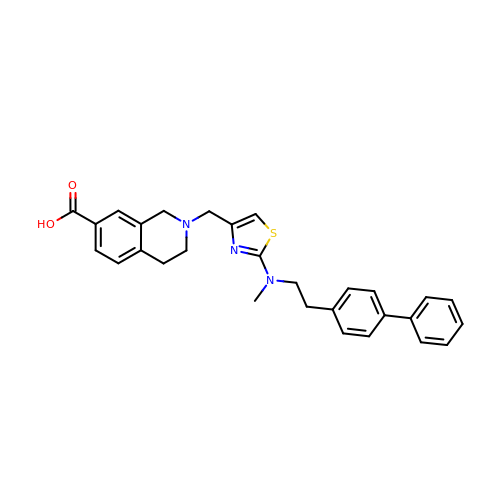2-[[2-[methyl-[2-(4-phenylphenyl)ethyl]amino]-1,3-thiazol-4-yl]methyl]-3,4-dihydro-1~{H}-isoquinoline-7-carboxylic acid | C29 H29 N3 O2 S | PZAXAHOHIQYROI-UHFFFAOYSA-N>[2x]GHMAKKTYDLLFKLLLIGDSGVGKTCVLFRFSDDAFNTTFISTIGIDFKIKTVELQGKKIKLQIWDTA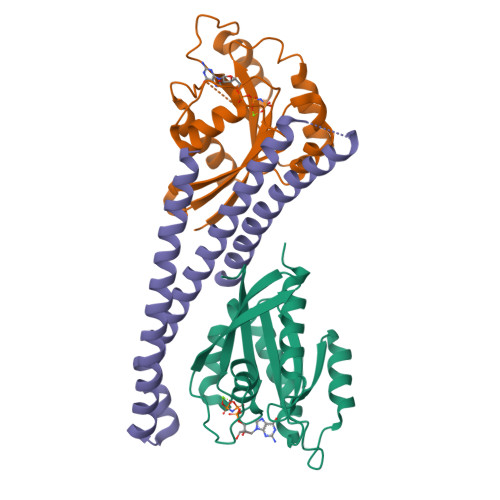GQERFHTITTSYYRGAMGIMLVYDITNGKSFENISKWLRNIDEHANEDVERMLLGNKCDMDDKRVVPKGKGEQIAREHGIRFFETSAKANINIEKAFLTLAEDILRKTP;> GHMKEEEMKRFCKAQTIQRRLNEIEAALRELEAEGVKLELALRRQSSSPEQQKKLWVGQLLQLVDKKNSLVAEEAELMITVQELNLEEKQWQLDQELRGYMNREENLKTAADRQAEDQVLRKLVDLVNQRDALIRFQEERRLSELALGTGAQG By combining microcrystal electron diffraction with native mass spectrometry (ED-MS), we develop an approach to rapidly and accurately determine structures of biosynthetic or clinically relevant ligands bound to enzymes. We demonstrate this approach with the model protein lysozyme bound to its noncovalent ligand N,N′,N″-triacetylchitotriose (ACT), then use the cysteine protease papain as a scaffold on which to bind a panel of both known and potential inhibitors, including the epoxide-based covalent cysteine protease inhibitor E-64 (27), its commercially available chemical analogs, and analogs generated by biosynthetic reaction. Last, we extend the ED-MS workflow to interrogate crystals of the β-lactamase enzyme, CTX-M-14, which imparts resistance to β-lactam-containing antibiotics by hydrolyzing their four-membered ring structural motif. Overall, our results demonstrate that structures of protein–ligand complexes can be obtained directly from microcrystal slurries by ED-MS, with unambiguous confirmation of the identity of the bound ligands.

We next interrogated ligand interactions of the cysteine protease papain, as isolated from papaya latex. Papain crystals were readily grown and cocrystallized or soaked with target ligands for MicroED analysis. Mass spectra acquired from apo papain crystals harvested from a TEM grid showed masses corresponding to the protein with both a doubly oxidized, sulfinic acid form (+32 Da) of its catalytic residue Cys25, and a reduced form of the protein. The assignment of this oxidation state is substantiated by its resistance to reduction with dithiothreitol (DTT) or tris(2-carboxyethyl)phospine (TCEP), unlike other +32 Da modifications such as persulfides, which would be reduced under these conditions.

> IPEYVDWRQKGAVTPVKNQGSCGSCWAFSAVVTIEGIIKIRTGNLNEYSEQELLDCDRRSYGCNGGYPWSALQLVAQYGIHYRNTYPYEGVQRYCRSREKGPYAAKTDGVRQVQPYNEGALLYSIANQPVSVVLEAAGKDFQLYRGGIFVGPCGNKVDHAVAAVGYGPNYILIKNSWGTGWGENGYIRIKRGTGNSYGVCGLYTSSFYPVKN>MMMASKDATSSVDGASGAGQLVPEVNASDPLAMDPVAGSSTAVATAGQVNPIDPWIINNFVQAPQGEFTISPNNTPGDVLFDLSLGPHLNPFLLHLSQMYNGWVGNMRVRIMLAGCAFTAGKIIVSCIPPGFGSHNLTIAQATLFPHVIADVRTLDPIEVPLEDVRNVLFHNNDRNQQTMRLVCMLYTPLRTCGGTGDSFVVAGRVMTCPSPDFNFLFLVPPTVEQKTRPFTLPNLPLSSLSNSRAPLPISSMGISPDNVQSVQFQNGRCTLDGRLVGTTPVSLSHVAKIRGTSNGTVINLTELDGTPFHPFEGPAPIGFPDLGGCDWHINMTQFGHSSQTQYDVDTTPDTFVPHLGSIQANGIGSGNYVGVLSWISPPSHPSGSQVDLWKIPNYGSSITEATHLAPSVYPPGFGEVLVFFMSKMPGPGAYNLPCLLPQEYISHLASEQAPTVGEAALLHYVDPDTGRNLGEFKAYPDGFLTCVPNGASSGPQQLPINGVFVFVSWVSRFY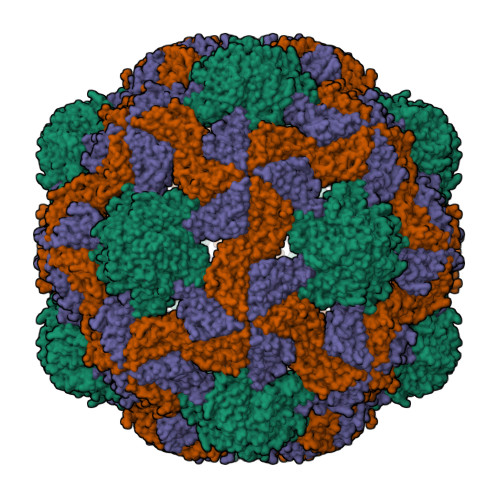QLKPVGTASSARGRLGLRR[3x]3-(N-HYDROXYACETAMIDO)-1-(3,4-DICHLOROPHENYL)PROPYLPHOSPHONIC ACID | C11 H14 Cl2 N O5 P | 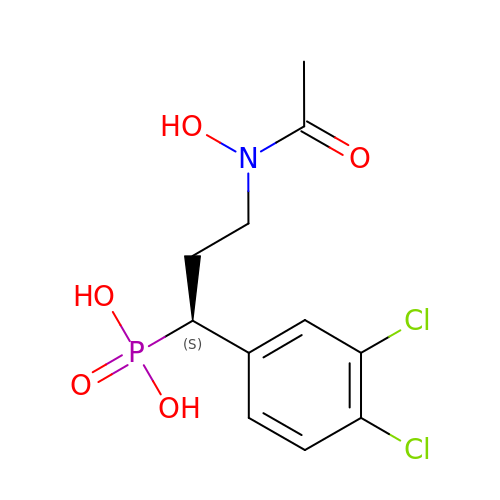ABGCTQYLJZGMBM-NSHDSACASA-N The human aldehyde dehydrogenase (ALDH) superfamily comprises 19 enzyme isoforms catalyzing the NAD(P)-dependent irreversible oxidation of aldehydes to their corresponding carboxylic acids. Cytosolic ALDH1A enzymes, and specifically the ALDH1A3 isoform, are good markers of cancer stem cells and have been implicated in carcinogenesis, chemoresistance and relapse. As previously observed in other members of the enzyme superfamily, each ALDH1A3 subunit is composed of three structural domains: a catalytic domain, a cofactor-binding domain and an oligomerization domain. At the intersection of the substrate- and cofactor-binding pockets sits a strictly conserved cysteine residue (Cys302, ALDH2 numbering), which is essential for catalysis, acting as the active-site nucleophile.

Each monomer of the ALDH1A3-NAD+ complex at 1.89-Å resolution contains one NAD+ molecule positioned in each of the cofactor-binding pockets. As expected, the NAD+ molecule in both subunits is accommodated showing its extended conformation (suitable for hydride transfer) and interacting directly with residues Thr178, Trp180, Lys204, Glu207, Ser258, and Glu411 through hydrogen bonds, and to other 20 residues via hydrophobic interactions (left). The adenosine ribose is held in position by hydrogen bonds between the 2′ and 3′ hydroxyl oxygen atoms and Lys204. Thr178, forming a hydrogen bond with the 3’ hydroxyl oxygen through its backbone oxygen, is unique to ALDH1A3 in comparison to other ALDH1A and ALDH2 enzymes, which have an Ile residue at this position for this purpose. Only Glu411 makes two hydrogen bonds to the 2′ and 3′ hydroxyl oxygen atoms of the nicotinamide ribose. The extended conformation of NAD+ allows hydride transfer between the substrate and the C4 atom of the nicotinamide ring of the cofactor, a necessary step in the catalytic mechanism which would not be possible with the NAD+ molecule in contracted form. The highest B-factor and lower occupancy values in the NAD+ molecule are detected in the nicotinamide moiety in both subunits A and B, whereas the adenosine moiety displays the best ordered part of the whole molecule. The ALDH1A3-NAD+ complex contains a PEG molecule (PEG1) close to the Cys314 residue in the substrate-binding pocket, with 6 and 4 oxygen atoms in monomers A and B, respectively. Also, in the substrate-binding pocket there is a small PEG molecule (PEG2) in the same place in all subunits. None of the two PEG1 molecules were covalently bound to the Cys314 residues, as it can be deduced from the distances between the Cys314-Sγ and the PEG1 atoms and also from the electron density shown in Fig. 5b. Next to Cys314 there is a water molecule that, as it will be shown later, will play an important role in the position of the PEG1 molecule in the ALDH1A3-ATP complex.

>[2x]HHHHHHLESTSLYKKAGMATANGAVENGQPDRKPPALPRPIRNLEVKFTKIFINNEWHESKSGKKFATCNPSTREQICEVEEGDKPDVDKAVEAAQVAFQRGSPWRRLDALSRGRLLHQLADLVERDRATLAALETMDTGKPFLHAFFIDLEGCIRTLRYFAGWADKIQGKTIPTDDNVVCFTRHEPIGVCGAITPWNFPLLMLVWKLAPALCCGNTMVLKPAEQTPLTALYLGSLIKEAGFPPGVVNIVPGFGPTVGAAISSHPQINKIAFTGSTEVGKLVKEAASRSNLKRVTLELGGKNPCIVCADADLDLAVECAHQGVFFNQGQCCTAASRVFVEEQVYSEFVRRSVEYAKKRPVGDPFDVKTEQGPQIDQKQFDKILELIESGKKEGAKLECGGSAMEDKGLFIKPTVFSEVTDNMRIAKEEIFGPVQPILKFKSIEEVIKRANSTDYGLTAAVFTKNLDKALKLASALESGTVWINCYNALYAQAPFGGFKMSGNGRELGEYALAEYTEVKTVTIKLGDKNP>GPHMSDHDYDVVIIGGGPAGSTMASYLAKAGVKCAVFEKELFEREHVGESLVPATTPVLLEIGVMEKIEKANFPKKFGAAWTSADSGPEDKMGFQGLDHDFRSAEILFNERKQEGVDRDFTFHVDRGKFDRILLEHAGSLGAKVFQGVEIADVEFLSPGNVIVNAKLGKRSVEIKAKMVVDASGRNVLLGRRLGLREKDPVFNQFAIHSWFDNFDRKSATQSPDKVDYIFIHFLPMTNTWVWQIPITETITSVGVVTQKQNYTNSDLTYEEFFWEAVKTRENLHDALKASEQVRPFKKEADYSYGMKEVCGDSFVLIGDAARFVDPIFSSGVSVALNSARIASGDIIEAVKNNDFSKSSFTHYEGMIRNGIKNWY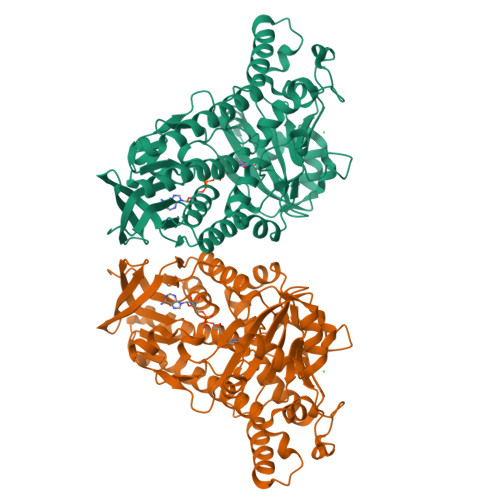EFITLYYRLNILFTAFVQDPRYRLDILQLLQGDVYSGKRLEVLDKMREIIAAVESDPEHLWHKYLGDMQVPTAKPAFEND[5x]>HHHHHHHHHHGTRRPELPDLAPEPRYAHIPVRIKEQVVGLLAWNNCSCESSGGGLPLPFQKQVRAIDLTKAFDPAELRAASATREQEFQAFLSRSQSPADQLLIAPANSPLQYPLQGVEVQPLRSILVPGLSLQAASGQEVYQVNLTASLGTWDVAGEVTGVTLTGEGQADLTLVSPGLDQLNRQLQLVTYSSRSYQTNTADTVRFSTEGHEAAFTIRIRHPPNPRLYPPGSLPQGAQYNISALVTIATKTFLRYDRLRALITSIRRFYPTVTVVIADDSDKPERVSGPYVEHYLMPFGKGWFAGRNLAVSQVTTKYVLWVDDDFVFTARTRLERLVDVLERTPLDLVGGAVREISGFATTYRQLLSVEPGAPGLGNCLRQRRGFHHELVGFPGCVVTDGVVNFFLARTDKVREVGFDPRLSRVAHLEFFLDGLGSLRVGSCSDVVVDHASKLKLPWTSRDAGAETYARYRYPGSLDESQMAKHRLLFFKHRLQCMTSQ[2x]

The localisation, activity and abundance of these glycosyltransferases is tightly regulated in cells to ensure different ganglioside levels are correctly maintained. β−1,4-N-Acetyl-Galactosaminyltransferase 1 (B4GALNT1) is a key enzyme of the ganglioside synthetic pathway, responsible for the synthesis of complex gangliosides. B4GALNT1 catalyses the transfer of an N-acetylgalactosamine (GalNac) from a Uridine diphosphate-GalNac donor (UDP-GalNac) onto the glycan headgroup of the ganglioside acceptor substrate. B4GALNT1 is a type-II membrane protein with a predicted domain structure consisting of a short (7-residue) N-terminal cytoplasmic sequence followed by a transmembrane helix and a 56 kDa lumenal domain.

The B4GALNT1 lumenal domain construct ΔN46 was crystallised for structure determination. Initial crystals possessed no ligands in the active site and diffracted to relatively low resolution, 3.6 Å. Microseeding during crystallisation combined with inclusion of manganese (Mn) in purification buffers improved the resolution of the structure to 2.94 Å for an apo-complex. In the apo structure of B4GALNT1, a long loop encompassing residues 486–510 was completely disordered. C Surface representation of the B4GALNT1 active site illustrating that in the Mn-bound (purple sphere) structure, without UDP ligands, the pocket is open and residues 486–510 are disordered.> MHHHHHHAVRASEISRVYEAYPEKKATLYFLVLGFLALIVGSLFGPFQALNYGNVDAYPLLKRLLPFVQSYYQGLTLHGVLNAIVFTQLFAQAIMVYLPARELNMRPNMGLMWLSWWMAFIGLVVFALPLLANEATVLYTFYPPLKGHWAFYLGASVFVLSTWVSIYIVLDLWRRWKAANPGKVTPLVTYMAVVFWLMWFLASLGLVLEFVLFLLPWSFGLVEGVDPLVARTLFWWTGHPIVYFWLLPAYAIIYTILPKQAGGKLVSDPMARLAFLLFLLLSTPVGFHHQFADPGIDPTWKMIHSVLTLFVAVPSLMTAFTVAASLEFAGRLRGGRGLFGWIRALPWDNPAFVAPVLGLLGFIPGGAGGIVNASFTLDYVVHNTAWVPGHFHLQVASLVTLTAMGSLYWLLPNLTGKPISDAQRRLGLAVVWLWFLGMMIMAVGLHWAGLLNVPRRAYIAQVPDAYPHAAVPMVFNVLAGIVLLVALLLFIYGLFSVLLSRERKPELAEAPLPFAEVISGPEDRRLV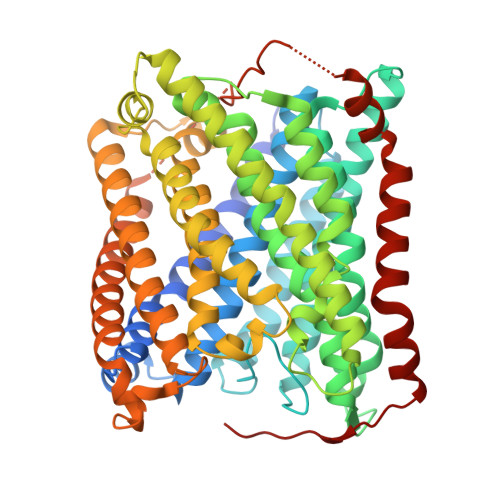LAMDRIGFWFAVAAILVVLAYGPTLVQLFGHLNPVPGWRLW> MILDVDYITEEGKPVIRLFKKENGKFKIEH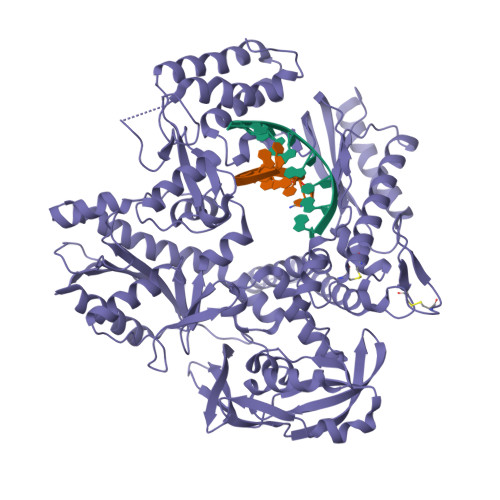DRTFRPYIYALLRDDSKIEEVKKITGERHGKIVRIVDVEKVEKKFLGKPITVWKLYLEHPQDQPTIREKVREHPAVVDIFEYDIPFAKRYLIDKGLIPMEGEEELKILAFAIATLYHEGEEFGKGPIIMISYADENEAKVITWKNIDLPYVEVVSSEREMIKRFLRIIREKDPDIIVTYNGDSFDFPYLAKRAEKLGIKLTIGRDGSEPKMQRIGDMTAVEVKGRIHFDLYHVITRTINLPTYTLEAVYEAIFGKPKEKVYADEIAKAWESGENLERVAKYSMEDAKATYELGKEFLPMEIQLSRLIGQPLWDVSRSSTGNLVEWFLLRKAYERNEVAPNKPSEEEYQRRLRESYTGGFVKEPEKGLWDDIVYLDFIALYPSIIITHNVSPDTLNLEGCKNYDIAPQVGHKFCKDIPGFIPSLLGHLLEERQKIKTKMKETQDPIEKILLDYRQKAIKLLANSFYGYYGYAKARWYCKECAESVTAWGRKYIELVWKELEEKFGFKVLYIDTDGLHATIPGGESEEIKKKALEFVKYINSKLPGLLELEYEGFYKRGFFVTKKRYAVIDEEGKVITRGLEIVRRDWSEIAKETQARVLETILKHGDVEEAVRIVKEVIQKLANYEIPPEKLAIYEQITRPLHEYKAIGPHVAVAKKLAAKGVKIKPGMVIGYIVLRGDGPISNRAILAEEYDPKKHKYDAEYYIENQVLPAVLRILEGFGYRKEDLRYQKTRQVGLTSWLNIKKS>GLPVEYLQVPSASMGRDIKVQFQGGGPHAVYLLDGLRAQDDYNGWDINTPAFEEYYQSGLSVIMPVGGQSSFYTDWYQPSQSNGQNYTYKWETFLTREMPAWLQANKGVSPTGNAAVGLSMSGGSALILAAYYPQQFPYAASLSGFLNPSESWWPTLIGLAM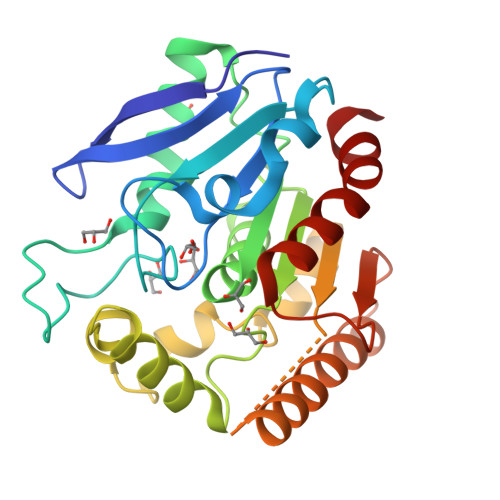NDSGGYNANSMWGPSSDPAWKRNDPMVQIPRLVANNTRIWVYCGNGTPSDLGGDNIPAKFLEGLTLRTNQTFRDTYAADGGRNGVFNFPPNGTHSWPYWNEQLVAMKADIQHVLNG[2x]5-{6-[(1-METHYLPIPERIDIN-4-YL)OXY]-1H-BENZIMIDAZOL-1-YL}-3-{(1R)-1-[2-(TRIFLUOROMETHYL)PHENYL]ETHOXY}THIOPHENE-2-CARBOXAMIDE | C27 H27 F3 N4 O3 S | 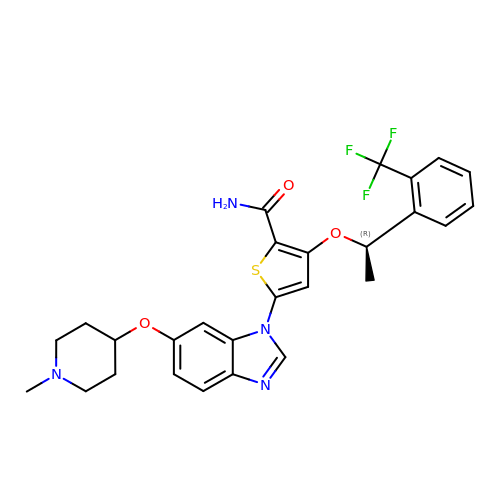SWIVJTVGOIXUKC-MRXNPFEDSA-N>[2x]MKKHHHHHHGKNNPDPTIYPVLDWNDIKFQDVIGEGNFGQVLKARIKKDGLRMDAAIKRMKEYASKDDHRDFAGELEVLCKLGHHPNIINLLGACEHRGYLYLAIEYAPHGNLLDFLRKSRVLETDPAFAIANSTASTLSSQQ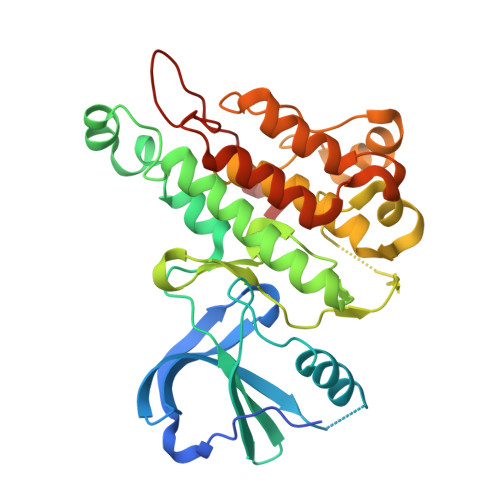LLHFAADVARGMDYLSQKQFIHRDLAARNILVGENYVAKIADFGLSRGQEVYVKKTMGRLPVRWMAIESLNYSVYTTNSDVWSYGVLLWEIVSLGGTPYCGMTCAELYEKLPQGYRLEKPLNCDDEVYDLMRQCWREKPYERPSFAQILVSLNRMLEERKTYVNTTLYEKFTYAGIDCSAEEAA3-(2-hydroxyphenyl)benzene-1,2-diol 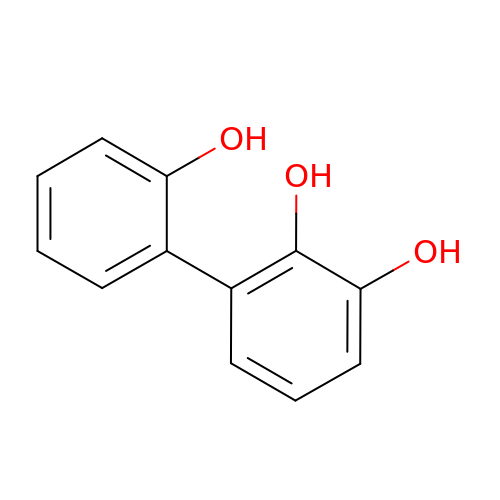| C12 H10 O3 | USBNIYMZDQVDSO-UHFFFAOYSA-N4-methyl-N-(6-phenoxypyridine-3-carbonyl)-L-leucine | C19 H22 N2 O4 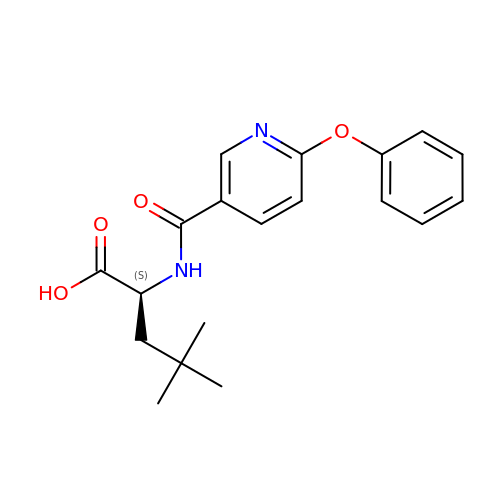| DASSWHWKVPKLEB-HNNXBMFYSA-N>[2x]AGRKVVVVGGGTGGATAAKYIKLADPSIEVTLIEPNTDYYTCYLSNEVIGGDRKLESIKHGYDGLRAHGIQVVHDSATGIDPDKKLVKTAGGAEFGYDRCVVAPGIELIYDKIEGYSEEAAAKLPHAWKAGEQTAILRKQLEDMADGGTVVIAPPAAPFRCPPGPYERASQVAYYLKAHKPMSKVIILDSSQTFSKQSQFSK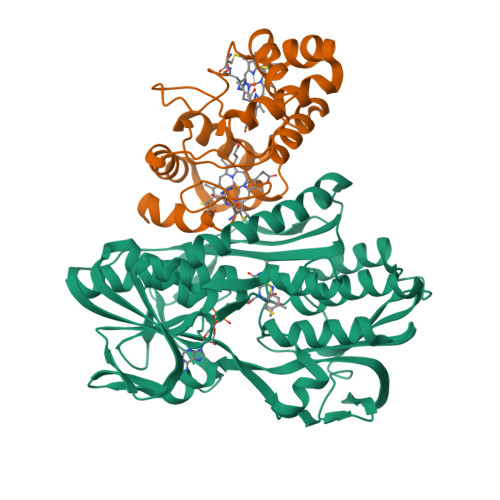GWERLYGFGTENAMIEWHPGPDSAVVKVDGGEMMVETAFGDEFKADVINLIPPQRAGKIAQIAGLTNDAGWCPVDIKTFESSIHKGIHVIGDASIANPMPKSGYSANSQGKVAAAAVVVLLKGEEPGTPSYLNTCYSILAPAYGISVAAIYRPNADGSAIESVPDSGGVTPVDAPDWVLEREVQYAYSWYNNIVHDTFG;>[2x]EPTAEMLTNNCAGCHGTHGNSVGPASPSIAQMDPMVFVEVMEGFKSGEIASTIMGRIAKGYSTADFEKMAGYFKQQTYQPAKQSFDTALADTGAKLHDKYCEKCHVEGGKPLADEEDYHILAGQWTPYLQYAMSDFREERRPMEKKMASKLRELLKAEGDAGLDALFAFYASQQ> MSYQNLVSEAGLTQKLLIHGDKELFQHELKTIFARNWLFLTHDSLIPSPGDYVKAKMGVDEVIVSRQNDGSVRAFLNVCRHRGKTLVHAEAGNAKGFVCGYHGWGYGSNGELQSVPFEKELYGDAIKKKCLGLKEVPRIESFHGFIYGCFDAEAPPLIDYLGDAAWYLEPTFKYSGGLELVGPPGKVVVKANWKSFAENFVGDGYHVGWTHAAALRAGQSVFSSIAGNAKLPPEGAGLQMTSKYGSGMGVFWGYYSGNFSADMIPDLMAFGAAKQEKLAKEIGDVRARIYRSFLNGTIFPNNSFLTGSAAFRVWNPIDENTTEVWTYAFVEKDMPEDLKRRVADAVQRSIGPAGFWESDDNENMETMSQNGKKYQSSNIDQIASLGFGKDVYGDECYPGVVGKSAIGETSYRGFYRAYQAHISSSNWAEF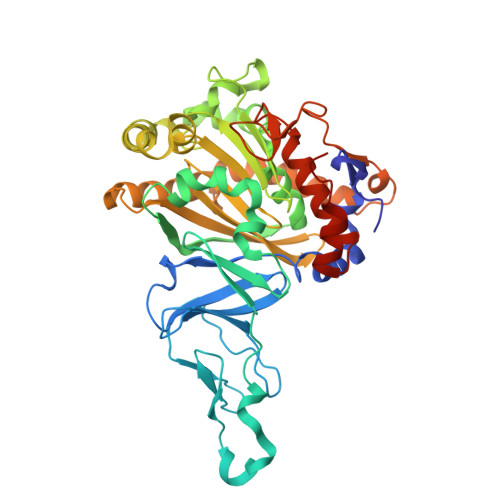ENASRNWHIEHTKTTDR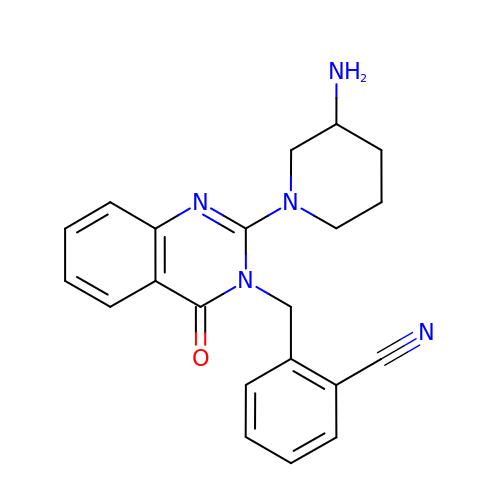2-({2-[(3R)-3-AMINOPIPERIDIN-1-YL]-4-OXOQUINAZOLIN-3(4H)-YL}METHYL)BENZONITRILE | C21 H21 N5 O | OYNURZXTLNNKAP-QGZVFWFLSA-N> MGRRQLARGRRYIGYDALKKNNVPCSRRGRSYYDCKKRRRNNP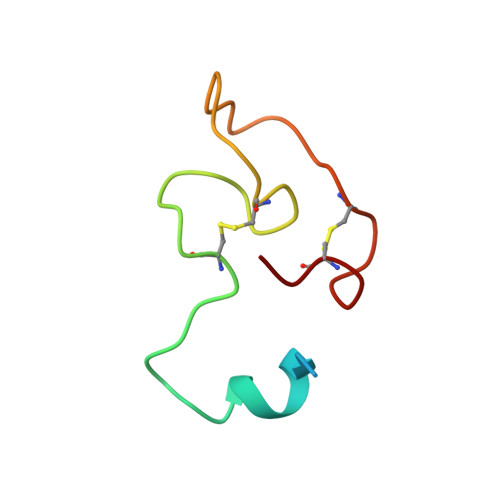YRRGCSAITHCYR> SALEVYTPKEIFVANG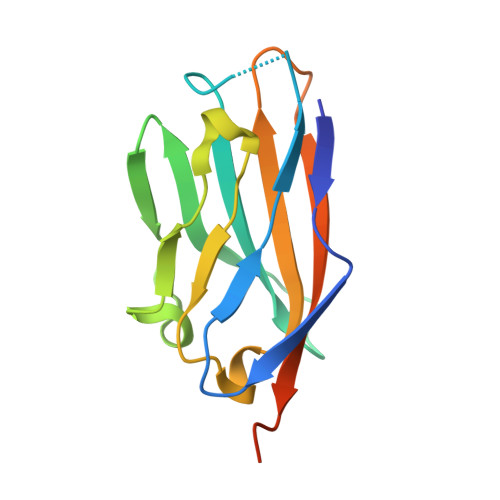TQGKLTCKFKSTSTTGGLTSVSWSFQPEGADTTVGFFHYSQGQVYLGNYPPFKDRISWAGDLDKKDASINIENMQFIHNGTYICDVKNPPDIVGKTSHIRLYVVEKENLPVLEHHHHHH We have recently identified interactions between two groups of Drosophila IgSF (immunoglobulin superfamily) cell adhesion molecules with properties closely matching a neuronal chemoaffinity function: 21 Dpr proteins, named after the founding member Defective proboscis extension response, selectively bind nine proteins, now called the Dpr-interacting proteins, or DIPs. All 21 Dprs and nine DIPs are predicted to contain two and three immunoglobulin (IG) domains, respectively. Our previous work identified the first IG domains, termed IG1, as the domains mediating the Dpr–DIP interaction by the formation of a pseudo-symmetric IG1-IG1 heterocomplex using the GFCC’C’ face of the immunoglobulin fold. Therefore, Dprs and DIPs are strong candidates for a synapse specification or targeting function.

During our crystallization trials, we also grew crystals and determined the structure of DIP-γ IG1 +2 in a monomeric state. This has allowed us to compare three structures containing DIP IG1 and IG2 domains and the relative orientations of these IG domains. In all structures, the two IG domains are in an extended conformation. The extended conformation is due to lack of linker sequences between the two IG domains in DIPs, which also holds true at the predicted DIP IG2-IG3 and the Dpr IG1-IG2 boundaries. However, despite the lack of sizeable linker sequences, the DIP IG1-IG2 domain boundary is flexible, allowing for movement of the DIP IG2 with respect to IG1. This is a result of the lack of stabilizing influences such as calcium ions found in cadherin domain boundaries or hydrogen bonds between the domains observed in SYG-1 and SYG-2. Lack of rigidity in Dprs and DIPs might indicate that they may not serve as signaling receptors directly and may not relay force or connect to cytoskeleton.

> SRLDPDPEFIGFINNVTYPAGREAILACSVRNLGKNKVGWLRASDQTVLALQGRVVTHNARISVMHQDMHTWKLKISKLRESDRGCYMCQINTSPMKKQVGCIDVQVPPDIINEESSADLAVQEGEDATLTCKATGNPQPRVTWRREDGEMILIRKPGSRELMKVESYNGSSLRLLRLERRQMGAYLCIASNDVPPAVSKRVSLSVHHHHHHH N,N~2~-bis(2-hydroxyethyl)glycinamide | C6 H14 N2 O3 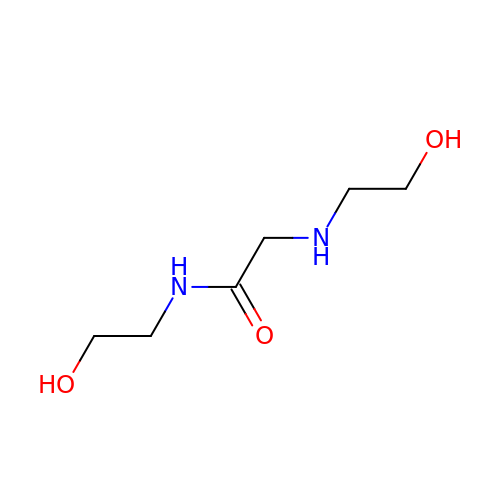| IXMVWXRQTPARRA-UHFFFAOYSA-N RET receptor tyrosine kinase plays vital developmental and neuroprotective roles in metazoans. GDNF family ligands (GFLs) when bound to cognate GFRα co-receptors recognize and activate RET stimulating its cytoplasmic kinase function. The bipartite GFL-GFR complexes are recognized by the RET receptor tyrosine kinase (RTK) forming ternary RET-GFL-GFR complexes (Cacalano et al., 1998; Durbec et al., 1996; Jing et al., 1996; Treanor et al., 1996). RET has four consecutive cadherin-like domains (CLD(1-4)) and a membrane-proximal cysteine-rich domain (CRD) in its extracellular domain (RETECD) (Anders et al., 2001).

Crystals were obtained for a zebrafish RET construct spanning residues 22–504 (zRET22-504) with glycosylation site mutations, N259Q, N308Q, N390Q, and N433Q (defined hereafter as zCLD(1-4)red.sug.). Diffraction data from these crystals led to a structure determination at 2.2 Å resolution. The crystals adopted the triclinic space group P1 and contained two molecules of CLD(1-4)red.sug. within the asymmetric unit. The final zCLD(1-4)red.sug. model contains residues 22–498 and includes 7 N-linked glycans well resolved in the electron density. The amino-terminal CLD1 is packed against CLD2 in a fold-over clamshell arrangement as anticipated from human RET, while CLD(2-4) forms a “C-shape”. The limited size of the CLD(2-3) interface is typical of a calcium-dependent cadherin domain pair, with three calcium ions (Ca-1/Ca-2/Ca-3) and their coordinating ligands dominating the interface. Differences in the CLD interface size indicate flexibility between CLD2 and CLD3 but rigidity between CLD3 and CLD4. Superimposing chain B onto chain A, aligned through CLD(1-2), reveals that the rigid CLD(3-4) module pivots about the CLD(2-3) calcium-binding site interface with a variation of 12.3°, which leads to a difference of 18.4 Å at the furthest point from the CLD(2-3) interface. Comparison of site 1 of zRET in both the crystal and cryo-EM structure reveals differences in the conformation of residues 288–298 from a CLD3 loop. In the absence of ligand, this loop packs against CLD3 core (loop “down” position) interacting with the β4 strand.

>[2x]LYFPQRLYTENIYVGQQQGSPLLQVISMREFPTERPYFFLCSHRDAFTSWFHIDEASGVLYLNKTLEWSDFSSLRSGSVRSPKDLTLKVGVSSTPPMKVMCTILPTVEVKLSFINDTAPSCGQVELSTLCFPEKISNPHITENREPGALRQLRRFTHMSICPNYTISYGVVAGSSVPFAVDDSTSELVVTAQVDREEKEVYHLDIVCMVRTERNLEEVFRSLHVNIYDEDDNSPYVQGTDTEDVLVEFDRSEGTVFGTLFVYDRDTTPVYPTNQVQNKLVGTLMTQDSWIKNNFAIEHKFREEKAIFGNVRGTVHEYKLKLSQNLSVTEQRSFLLGYLVNDTTFPGPEGTVLLHFNVTVLPVPIRFSQVTYSFTVSQKATTYSQIGKVCVENCQKFKGIDVTYQLEIVDRQITAEAQSCYWAVSLAQNPNDNTGVLYVNDTKVLRRPECQELEYVVIAQEQQNKLQAKTQLTVSFQGEAD>MTADELVFFVNGKKVVEKNADPETTLLVYLRRKLGLCGTKLGCGEGGCGACTVMISKYDRLQNKIVHFSVNACLAPICSLHHVAVTTVEGIGNTQKLHPVQERIARSHGSQCGFCTPGIVMSMYTLLRNQPEPTVEEIENAFQGNLCRCTGYRPILQGFRTFAKDGGCCGGSGNNPNCCMNQTKDQTVSLSPSLFNPEDFKPLDPTQEPIFPPELLRLKDTPQKKLRFEGERVTWIQASTMEELLDLKAQHPDAKLVVGNTEIGIEMKFKNMLFPLIVCPAWIPELNSVVHGPEGISFGASCPLSLVESVLAEEIAKLPEQKTEVFRGVMEQLRWFAGKQVKSVASIGGNIITASPISDLNPVFMASGAKLTLVSRGTRRTVRMDHTFFPGYRKTLLRPEEILLSIEIPYSKEGEFFSAFKQASRREDDIAKVTSGMRVLFKPGTIEVQELSLCFGGMADRTISALKTTPKQLSKSWNEELLQSVCAGLAE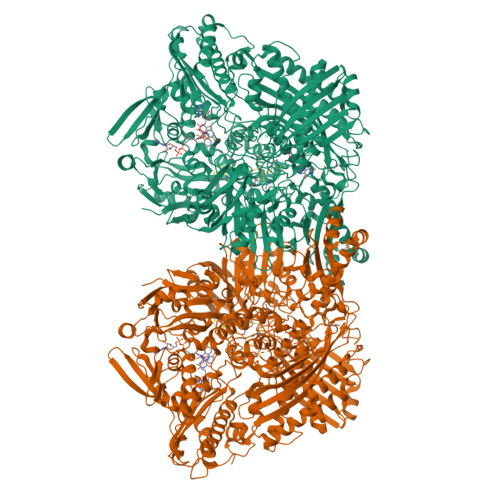ELQLAPDAPGGMVEFRRTLTLSFFFKFYLTVLQKLGRADLEDMAGKLDPTFASATLLFQKDPPANVQLFQEVPKDQSEEDMVGRPLPHLAANMQASGEAVYCDDIPRYENELSLRLVTSTRAHAKITSIDTSEAKKVPGFVCFLTAEDVPNSNATGLFNDETVFAKDEVTCVGHIIGAVVADTPEHAQRAARGVKITYEDLPAIITIQDAINNNSFYGSEIKIEKGDLKKGFSEADNVVSGELYIGGQEHFYLETNCTIAVPKGEAGEMELFVSTQNTMKTQSFVAKMLGVPDNRIVVRVKRMGGGFGGKETRSTVVSTALALAAHKTGRPVRCMLDRDEDMLITGGRHPFLAKYKVGFMKTGTVVALEVAHFSNGGNTEDLSRSIMERALFHMDNAYKIPNIRGTGRICKTNLPSNTAFRGFGGPQGMLIAEYWMSEVAITCGLPAEEVRRKNMYKEGDLTHFNQKLEGFTLPRCWDECIASSQYLARKREVEKFNRENRWKKRGLCIIPTKFGISFTLPFLNQGGALVHVYTDGSVLLTHGGTEMGQGLHTKMVQVASRALKIPTSKIHISETSTNTVPNTSPTAASASADLNGQGVYEACQTILKRLEPFKKKKPTGPWEAWVMDAYTSAVSLSATGFYKTPNLGYSFETNSGNPFHYFSYGVACSEVEIDCLTGDHKNLRTDIVMDVGSSLNPAIDIGQVEGAFVQGLGLFTMEELHYSPEGSLHTRGPSTYKIPAFGSIPIEFRVSLLRDCPNKRAIYASKAVGEPPLFLASSIFFAIKDAIRAARAQHGDNAKQLFQLDSPATPEKIRNACVDQFTTLCVTGVPENSKSWSVRI[2x]During energy production in Desulfitobacterium hafniense, MtgA catalyzes the methyl transfer from methylcobalamin (Cbl‐CH3) to THF in the catabolism of glycine betaine (GB). Despite its lack of sequence identity with known structures, we could show that MtgA forms a homodimeric complex of two TIM barrels. The topology of each subunit is characterized by a funnel of eight parallel β‐sheets connected by α‐helices on the outside that form a complex of two perpendicularly oriented TIM barrels. The active‐site cavity is located inside the hydrophilic core of each barrel.

Herein, we present X‐ray structures of THF‐ and THF‐CH3‐bound MtgA that allow us atomic insights into the reaction trajectory of this catalyst. In contrast to substrate‐bound MtgA, the entire cofactor is defined in the MtgA:THF‐CH3 complex depicting extensive coordination within the amino acid environment in a rigid manner. The overall binding motif of the pterin ring remains similar to the substrate‐bound structure. However, the THF benzoate moiety is now involved in a π‐stacking network including Tyr230, Phe243, Phe251, and Trp272 on one side, as well as Tyr35 and His38 on the other. While the functional groups of the THF tail engage water‐coupled hydrogen bonding interactions with adjacent residues, the terminal γ‐carboxylate forms salt bridges with Arg236 that coordinate the cofactor in an extended conformation. Mutation of Arg236 to alanine resulted in impaired enzymatic activity, thus implying that fixation of the THF tail during methylation is involved in catalysis. Besides this fixation, the superposition of both ligand structures illustrates a rotation of the pterin moiety during the reaction of approximately 35°. In contrast, the benzoate group of THF‐CH3 displaces the carboxamide side chain of Asn227 by 2 Å (red double arrow). As planar sp2 hybridization would be expected in this position of the final product THF‐CH3, the X‐ray structure must depict a trapped protonated reaction intermediate. On the other hand, the WT MtgA:THF‐CH3 structure illustrates an intermediate that forms immediately after CH3 transfer from Cbl‐CH3 to THF.

>GSFKFTAQQHVYDINGVKVGGQPGEYPTVLIGSIFYRGHKIVSDGQKGIFDKDAAKALLDQEAELSAETGNPFIIDVLGESVEALTKYVEFILENTTAPFLLDSISPDVRVGALKNLGKDPEIQKRLIYNSIEEHYTEEELAAIKEAGLKTAVILAFSKKALKPNARIDLLQGKDDKEGLIAAAKRAGIEQFLVDPGVLDVASNSWTTEAINVVKEQFGYPGGCAPSNAVYLWKKMRSKGTPFFEVAGAAVFTYPITQGADFILYGPMMNAPWVYRAIATTDAMIAYNNKLTGVKMGTTEHPLLKIF[4x]> LEK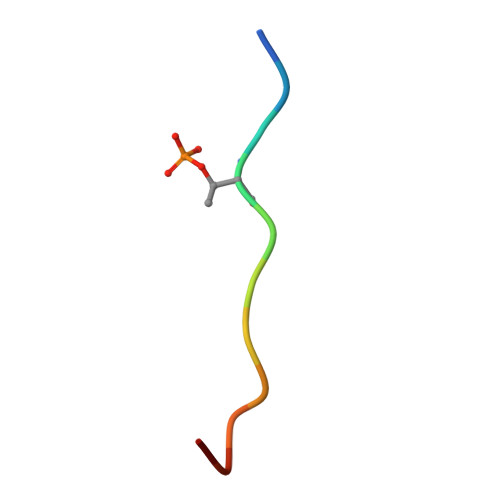TSIVASDTX>[2x]MSTGDFLTKGIELVQKAI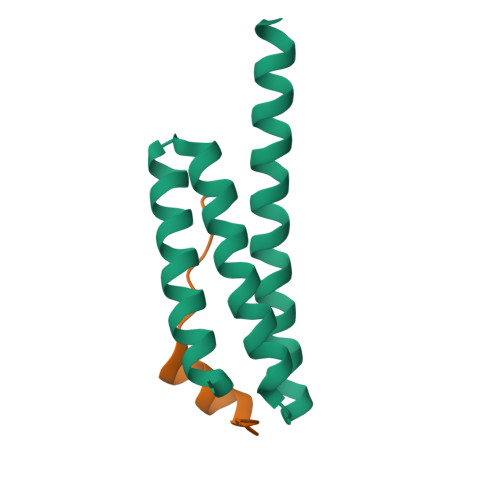DLDTATQYEEAYTAYYNGLDYLMLALKYEKNPKSKDLIRAKFTEYLNRAEQLKKHLESEEANAA;>[2x]ENYSNTDPEELLRKHVFPSVPK ABCB10, a member of ABC transporter superfamily that locates in the inner membrane of mitochondria, plays crucial roles in hemoglobin synthesis, antioxidative stress and stabilization of the iron transporter mitoferrin-1. Recently, it was found that ABCB10 is a mitochondrial biliverdin exporter. Each monomer contains two parts, the transmembrane domains (TMDs) and the nucleotide binding domains (NBDs). Here we report the cryo-EM structures of ABCB10 in apo (ABCB10-apo) and biliverdin-bound form (ABCB10-BV) at 3.67 Å and 2.85 Å resolution, respectively.

Unexpectedly, we obtained both BV-free (ABCB10-apo) and BV-bound (ABCB10-BV) structures at 3.67 Å and 2.85 Å resolution cryo-electron microscopy (EM) maps from a single data set after data processing, respectively. The final model of ABCB10-apo encompasses residues from 156 to 724, missing the C-terminal 14 residues and 528-532 in NBD. ABCB10-apo dimer adopts an inward-facing, wide-open conformation, awaiting the transport substrate. However, ABCB10-apo exhibits a more wide-open conformation than other three, suggesting that either ATP or BV can trigger the conformational changes. ABCB10-apo holds a much bigger pocket for substrate, indicating that it is more competent for substrate-binding than others. ABCB10-apo may thus represent the initial stage of substrate export. The ATPase sites are about 30 Å apart in apo form, a distance far beyond the reach of ATP molecules, which is consistent with the low basal ATPase activity observed before. Our ABCB10-apo structure is consistent with this model in that TMH4-5 are swapped in the inward-facing dimer. Our ABCB10-apo structure which is in wide-open conformation may represent the initial stage of export, namely apo form, because it contains a much bigger pocket and is thus more susceptible to substrates. Although it is possible that cholesterol is located there because that region of ABCB10-BV provides an environment that accommodates the interaction with hydrophobic and amphipatic molecules. It might be also the reason that cholesterol can be seen in ABCB10-BV but not in ABCB10-Apo.

> MAGLPEARKLLGLAYPERRRLAAAVGFLTMSSVISMSAPFFLGKIIDVIYTNPTVDYSDNLTRLCLGLSAVFLCGAAANAIRVYLMQTSGQRIVNRLRTSLFSSILRQEVAFFDKTRTGELINRLSSDTALLGRSVTENLSDGLRAGAQASVGISMMFFVSPNLATFVLSVVPPVSIIAVIYGRYLRKLTKVTQDSLAQATQLAEERIGNVRTVRAFGKEMTEIEKYASKVDHVMQLARKEAFARAGFFGATGLSGNLIVLSVLYKGGLLMGSAHMTVGELSSFLMYAFWVGISIGGLSSFYSELMKGLGAGGRLWELLEREPKLPFNEGVILNEKSFQGALEFKNVHFAYPARPEVPIFQDFSLSIPSGSVTALVGPSGSGKSTVLSLLLRLYDPASGTISLDGHDIRQLNPVWLRSKIGTVSQEPILFSCSIAENIAYGADDPSSVTAEEIQRVAEVANAVAFIRNFPQGFNTVVGEKGVLLSGGQKQRIAIARALLKNPKILLLDQATSALDAENEYLVQEALDRLMDGRTVLVIAHRLSTIKNANMVAVLDQGKITEYGKHEELLSKPNGIYRKLMNKQSFISAENLYFQGDYKDDDDKHHHHHHHHHH>[2x]GGC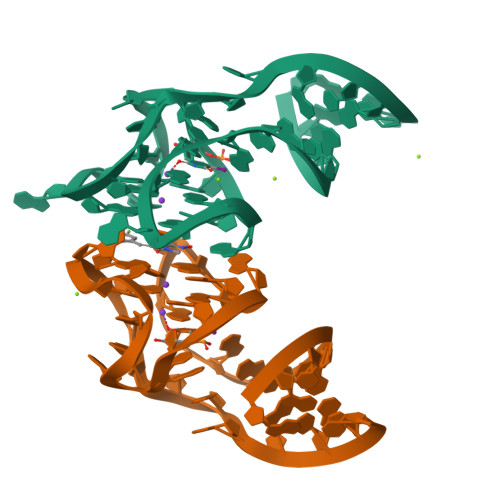GCGAGGAAGGAGGUCUGAGGAGGUCACUGCGCC> GSGIKSNPSKRHRDRLNTELDRLASLLPFPQDVINKLDKLSVLRLSVSYLRAKSFFDVALKSTPADRNGGQDQCRAQIRDWQDLQEGEFLLQALNGFVLVVTADALVFYASSTIQDYLGFQQSDVIHQSVYELIHTEDRAEFQRQLHWALNPDSAQGVDEAHGPPQAAVYYTPDQLPPENASFMERCFRCRLRCLLDNSSGFLAMNFQGRLKYLHGQNKKGKDGALLPPQLALFA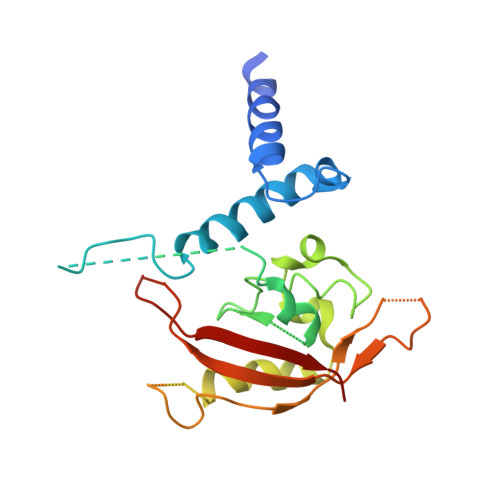IATPLQ> MLRLTQAVLRVQSHQKKRAQHPNAGTRFGRVYNRGFVRYGFGGFGMSVYSSKKDRTFKVMPVPPPPPATTAVEQRDDFADNRGLSATTRTLSPTFRMFALEDGGVLVSHPSHAQIMRWNQRVHTEEGKAANSTVMDEYVNSRIQAIIADNTIENTSLSQWRKAHMWNVIKSHGKLQRRWGTPDFVMGARSTLYN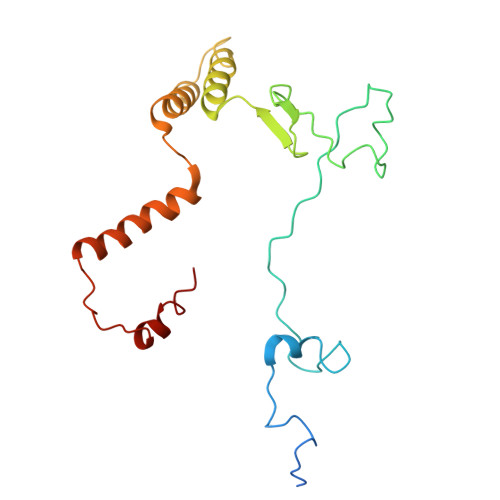N> MGPGLLYNHAAKTAVNGIDRSTEGTNVSARLCNNISAVTFVSKYKAVCQPIADQLDLPVENLLGLAAQESQYGTGRIARELNNYFSMHAPAPLQIGAEAPLGNASIKVAKFDSFQKSAQSFASSFGTAVRGQRDPMAFAQALVRSGYNTGNAKTGGRDGFARYLADIIIAVRGRMAC;> GSHMATDSLQPARIK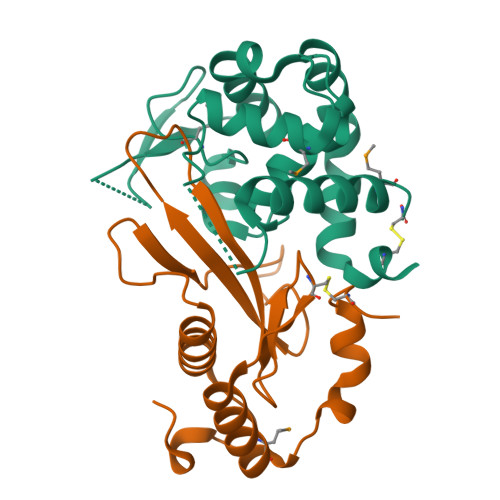DSGLTREQAEQVLRVALKHQDYQLQRPGVFIDGDLQDENGKPPHPGYYDFSLGYNDPKAGATEYWGLFSVSLNTGDTWEINSCKRLDGAELRALQRRVMARTGKSLADEKSQREGLGCEDQQ>[8x]MRLPILIINFKAYGEAAGKRAVELAKAAERAARELGVNIVVAPNHLELGLVSQSVDIPVYAQGADVEAGGAHTAHVSLE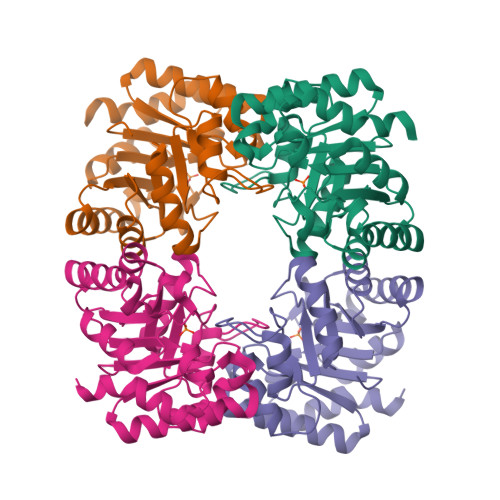NIKEAGGSGVILNHSEAPLKLNDLARLVAKAKSLGLDVVVCAPDPRTSLAAAALGPHAVAVEPPELIGTGRAVSRYKPEAIVETVGLVSRHFPEVSVITGAGIESGDDVAAALRLGTRGVLLASAAVKAKDPYAKIVELAKPLSELR>[10x]APQSITELCSEYHNTQIYTINDKILSYTESMAGKREMVIITFKSGATFQVE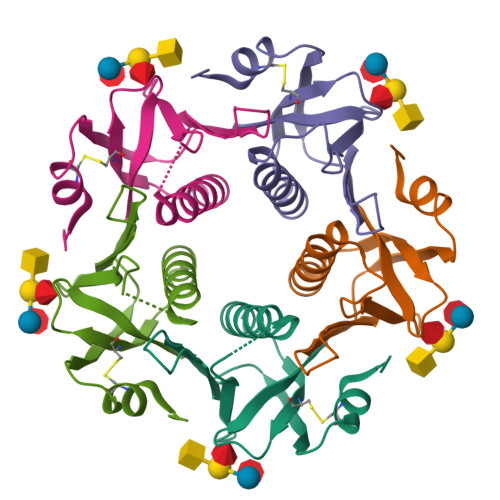VPGSQHIDSQKKAIERMKDTLRITYLTETKIDKLCVWNNKTPNSIAAISMEK Phylogenetic analysis shows that, within the rhodopsin superfamily, viral rhodopsins form a monophyletic family that consists of two distinct groups, VR1 and VR2. Here we present the results of a comprehensive structure-function study of two homologous proteins (61% sequence similarity) from the VR1 group, OLPVR1 (ADX06642.1), and VirChR1 (TARA-146-SRF-0.22-3-C376786_1). In this work, we demonstrate that VR1 rhodopsins are Na+/K+ selective light-gated ion channels that are inhibited by divalent cations. VirChR1s have proteorhodopsin-like architecture with short extracellular loops and share several structural features, such as membrane-associated ICL2 helix and an unconventional TM6-TM7 orientation.

Here, we present a high-resolution structure of another VR1 protein, OLPVR1, at 1.4 Å resolution. Type A rhombic crystals were grown at pH 8.0 using the monopalmitolein (MP) host lipid matrix and have the P21212 space group with one protein molecule in the asymmetric unit. Type A and type B crystals resulted in the obtaining of the OLPVR1 structures at the resolution of 1.4 and 1.6 Å, respectively. OLPVR1 molecules are nearly identical in both structures (root mean square deviation (RMSD) less than 0.2 Å), so hereafter, we refer to the structure from type A crystals as it has the highest resolution. The OLPVR1 protein (residues 2–223), all-trans retinal (ATR) covalently bound to K204 (K257 in CrChR28), 9 lipid molecules, and 107 water molecules are clearly resolved in the electron density maps. 2Fo–Fc electron density maps at 1.4 Å reveal two alternative conformations of the retinal in the region of the β-ionone ring. At the same time, the configuration near the Schiff base in both of them is all-trans 15-anti. Strikingly different from other rhodopsins, the intracellular parts of TM6 and TM7 helices of OLPVR1 are significantly moved apart from each other far enough to form a pore. The pore is located at about 8 Å from the cytoplasmic side of the lipid membrane border and connects the inside of the protein with the groove on its surface, which leads further to the intracellular bulk. Surprisingly, in our structure, the groove and a part of the pore are occupied with a fragment of the lipid molecule, a host lipid of the crystallization matrix (MP and MO in case of 1.4 and 1.6 Å structures, respectively), which is likely to be a crystallization artifact and is discussed in more details in the Supplementary Notes.

> MDNIIMTAYISIFVQIITAIISVYGLFIPLNFKDIILREILILELIVQIIEFIFYIWLIITLQSINEDITYVRYFDWVLTTPVMLLTTVYFFEYMNSDDGIRKKEINDRDYVYLFYICLSNFFMLLIGYLGETKQINKMLTLFGGSFFLFLTFYLLYVKYTKENWMNYIVFYFMFLVWFLYGFAFMFPFSIKNQMYNILDIVSKNIYSIFIFIVILNQSYKLLLEHHHHHH> SEVVSFSFTKFNPNPKDIILQGDALVTSKGKLQLTKVKDGKPVDHSLGRALYAAPIHIWDDSTDRVASFATSFSFVVEAPDESKTADGIAFFLAPPDTQPQKDGGFLGLFNDSNKSIQTVAVEFDTFSNTWDPSARHIGINVNSIESMKYVKWGWENGKVANVYISYEASTKTLTASLTYPSNATSYIVSANVDLKSALPEWVRVGFSATSGLSRDH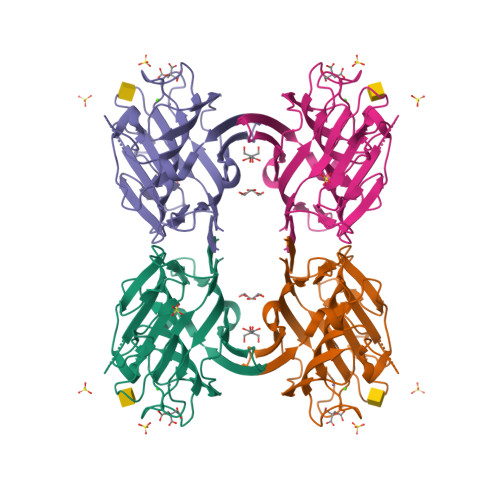VETHDVLDWSFTSTLQAPSDDSN>[2x]GPMTDWPVYHRIDGPIVMIGFGSIGRGTLPLIERHFAFDRSKLVVIDPSDEARKLAEAR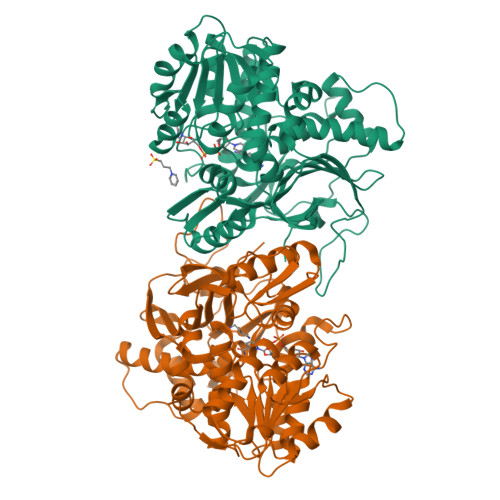GVRFIQQAVTRDNYRELLVPLLTAGPGQGFCVNLSVDTSSLDIMELARENGALYIDTVVEPWLGFYFDPDLKPEARSNYALRETVLAARRNKPGGTTAVSCCGANPGMVSWFVKQALVNLAADLGVTGEEPTTREEWARLAMDLGVKGIHIAERDTQRASFPKPFDVFVNTWSVEGFVSEGLQPAELGWGTFERWMPDNARGHDSGCGAGIYLLQPGANTRVRSWTPTAMAQYGFLVTHNESISIADFLTVRDAAGQAVYRPTCHYAYHPCNDAVLSLHEMFGSGKRQSDWRILDETEIVDGIDELGVLLYGHGKNAYWYGSQLSIEETRRIAPDQNATGLQVSSAVLAGMVWALENPNAGIVEADDLDFRRCLEVQTPYLGPVVGVYTDWTPLAGRPGLFPEDIDTSDPWQFRNVLVRD> MGAQVSSQKVGAHENSNRAYGGSTINYTTINYYRDSASNAASKQDFAQDPSKFTEPVKDVLIKTAPTLNSPNIEACGYSDRVMQLTLGNSTITTQEAANSVVAYGRWPEYIKDSEANPVDQPTEPAVAACRFYTLDTVTWRK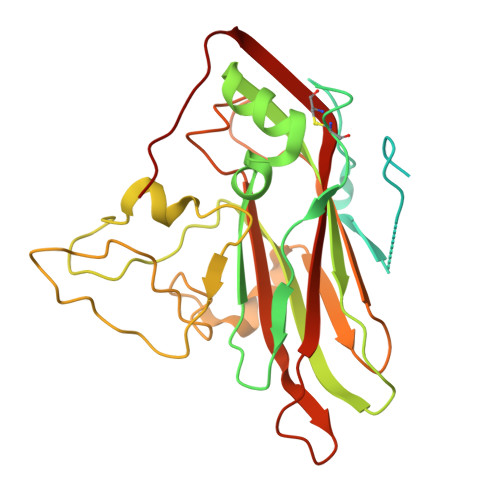ESRGWWWKLPDALKDMGLFGQNMFYHYLGRAGYTVHVQCNASKFHQGALGVFAVPEMCLAGDSTTHMFTKYENANPGEKGGEFKGSFTLDTNATNPARNFCPVDYLFGSGVLAGNAFVYPHQIINLRTNNCATLVLPYVNSLSIDSMTKHNNWGIAILPLAPLDFATESSTEIPITLTIAPMCCEFNGLRNITVPRTQ>MVTVVEEVDHLPIYDLDPKLEEFKDHFNYRIKRYLDQKCLIEKHEGGLEEFSKGYLKFGINTVDGATIYREWAPAAQEAQLIGEFNNWNGAKHKMEKDKFGIWSIKISHVNGKPAIPHNSKVKFRFRHGGGAWVDRIPAWIRYATFDASKFGAPYDGVHWDPPACERYVFKHPRPPKPDAPRIYEAHVGMSGEEPEVSTYREFADNVLPRIRANNYNTVQLMAIMEHSYYASFGYHVTNFFAVSSRSGTPEDLKYLVDKAHSLGLRVLMDVVHSHASNNVTDGLNGYDVGQNTHESYFHTGDRGYHKLWDSRLFNYANWEVLRFLLSNLRYWMDEFMFDGFRFDGVTSMLYHHHGINKGFTGNYKEYFSLDTDVDAIVYMMLANHLMHKLLPEATIVAQDVSGMPVLCRPVDEGGVGFDFRLAMAIPDRWIDYLKNKEDRKWSMSEIVQTLTNRRYTEKCIAYAESHDQSIVGDKTIAFLLMDKEMYTGMSDLQPASPTINRGIALQKMIHFITMALGGDGYLNFMGNEFGHPEWIDFPREGNNWSYDKCRRQWSLVDTDHLRYKYMNAFD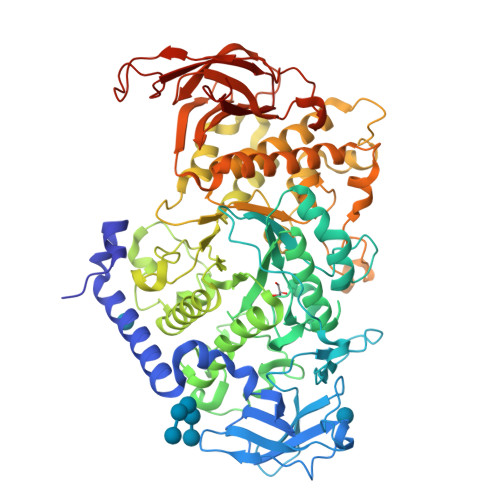QAMNALEEEFSFLSSSKQIVSDMNEKDKVIVFERGDLVFVFNFHPNKTYKGYKVGCDLPGKYRVALDSDALVFGGHGRVGHDVDHFTSPEGMPGVPETNFNNRPNSFKVLSPPRTCVAYYRVDEDREELRR[2x]> AVSSSRGGITVLTHSELSAEIGVTDSIVVSSELVMPYTVGTWLRGVAA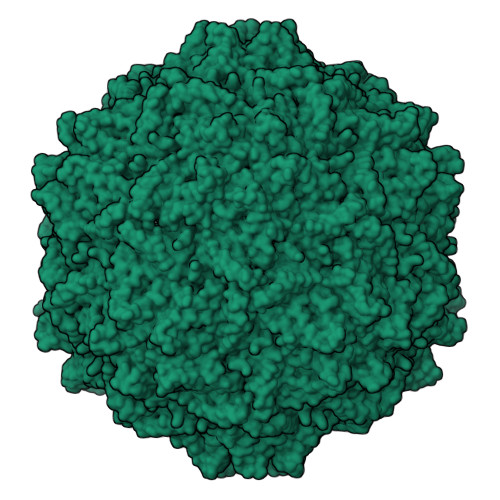NWSKYSWLSVRYTYIPSCPSSTAGSIHMGFQYNMANTVPVSVNQLSNLRGYVSGQVWSGSAGLCFINGTRCSDTSTAISTTLDVSKLGKKWYPYKTSADYATAVGVDVNIATPLVPARLVIALLDGSSSTAVAAGRIYCTYTIQMIEPTASALNN> NPVENYIDEVLNEVLVVPNIKESHHTTSNSAPLLDAAETGHTSNVQPEDAIETRYVITSQTRDEMSIESFLGRSGCVHISRIKVDYTDYNGQDINFTKWKITLQEMAQIRRKFELFTYVRFDSEITLVPCIAGRGDDIGHIVMQYMYVPPGAPIPSKRNDFSWQSGTNMSIFWQHGQPFPRFSIPFLSIASAYYMFYDGYDGDNTSSKYGSVVTNDMGTICSRIVTEKQK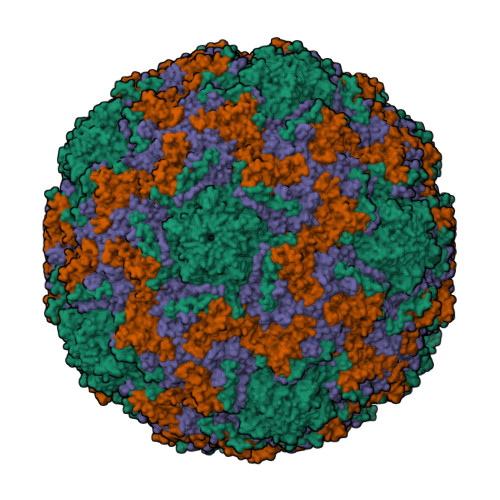LSVVITTHIYHKAKHTKAWCPRPPRAVPYTHSHVTNYMPETGDVTTAIVRRNTITTA;> SPSVEACGYSDRIMQITRGDSTISSDDVANAVVGYGVWPHYLTPQDATAINKPTQPDTSSNRFYTLESKHWNGSSKGWWWKLPDALKDMGIFGENMYYHFLGRSGYTVHVQCNASKFHQGTLLVAMIPEHQLASAKHGSVTAGYKLTHPGEAGRDVSQERDASLRQPSDDSWLNFDGTLLGNLLIFPHQFINLRSNNSATLIVPYVNAVPMDSMLRHNNWCLVIIPISPLRSETTSSNIVPITVSISPMCAEFSGARAKNIKQ;> GLPVYITPGSGQFMTTDDMQSPCALPWYHPTKEISIPGEVKNLIEMCQVDTLIPVNNVGNNVGNVSMYTVQLGNQTGMAQKVFSIKVDITSTPLATTLIGEIASYYTHWTGSLRFSFMFCGTANTTLKLLLAYTPPGIDEPTTRKDAMLGTHVVWDVGLQSTISLVVPWVSASHFRLTADNKYSMAGYITCWYQTNLVVPPSTPQTADMLCFVSACKDFCLRMARDTDLHIQSGPIEQ;> GAGVSRQNVGTHSTQNSVSNGSSLNYFNINYFKDAASSGASRLD>MNHKVHHHHHHMGADSVISFAKTLLGKPYVWGAEGPNSFDCSGFTQYVMKKSVGVSIPRVSRDQSKYGTYVNRGDLRSGDLVFFDTQGSNNGSVSHVGIYIGNGDMIHASSG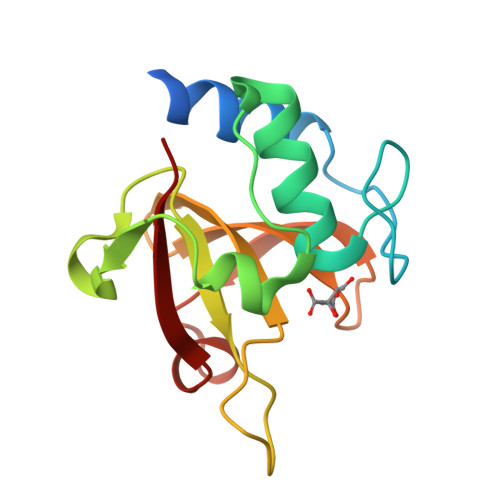SSKKVTISNINSSYYSSRYVNARRVL[4x]>[2x]MTPPHNYLAVIKVVGIGGGGVNAVNRMIEQGLKGVEFIAINTDAQALLMSDADVKLDVGRDSTRGLGAGADPEVGRKAAEDAKDEIEELLRGADMVFVTAGEGGGTGTGGAPVVASIARKLGAL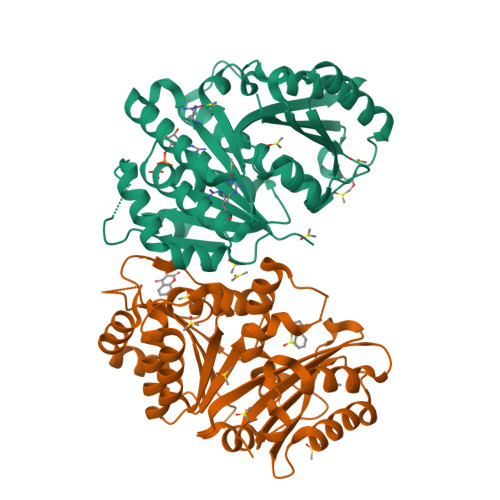TVGVVTRPFSFEGKRRSNQAENGIAALRESCDTLIVIPNDRLLQMGDAAVSLMDAFRSADEVLLNGVQGITDLITTPGLINVDFADVKGIMSGAGTALMGIGSARGEGRSLKAAEIAINSPLLEASMEGAQGVLMSIAGGSDLGLFEINEAASLVQDAAHPDANIIFGTVIDDSLGDEVRVTVIAAGFDV>MAPLATRQGKRPSKNLKARCSRKALHVNFKDMGWDDWIIAPLEYEAFHCEGLCEFPLRSHLEPTNHAVIQTLMNSMDPESTPPTCCVPTRLSPISILFIDSANNVVYKQYEDMVVESCGCR[2x];>[2x]ETGCNKALCASDVSKCLIQELCQCRPGEGNCSCCKECMLCLGALWDECCDCVGMCNPRNYSGTLEVLFQ

Twisted gastrulation (TWSG1) is an evolutionarily conserved secreted glycoprotein which controls signaling by Bone Morphogenetic Proteins (BMPs). TWSG1 binds BMPs and their antagonist Chordin to control BMP signaling during embryonic development, kidney regeneration and cancer. TWSG1 is composed of two distinct, disulfide-rich domains. The TWSG1 N-terminal domain occupies the BMP type 1 receptor binding site on BMPs, whereas the C-terminal domain binds to a Chordin family member.

To understand how TWSG1 interacts with BMP ligands, we determined the crystal structure of the TWSG1 NTD in complex with GDF5 at 1.96 Å resolution. The disulfide-linked GDF5 dimer binds to two TWSG1 NTD molecules that are related by a non-crystallographic pseudo two-fold axis (RMSD of 0.419 Å for 138 equivalent Cα atoms of the 1:1 TWSG1 NTD:GDF5 complexes). The two TWSG1 NTD molecules in the complex adopt a similar conformation compared to the apo TWSG1 NTD (0.33 Å for 38 equivalent Cα atoms), with the major variability observed in the loop connecting helices α1 and α2. The TWSG1 NTD binds to the finger region of GDF5 and interacts with both protomers of the GDF5 dimer. The TWSG1–GDF5 interface centers around helix α1 of TWSG1 sequestered between the two finger-like motifs and helix α3 of GDF5. The side chain of TWSG1 Ile40, at the core of this interface, inserts into the hydrophobic pocket of GDF5 formed by Trp414, Trp417, Val448, Ile449, Phe478, and Tyr490, and is shielded by a salt bridge between TWSG1 Glu42 and GDF5 Lys488. TWSG1–GDF5 interactions are mediated by two salt bridges (TWSG1 Lys28-GDF5 Glu434 and TWSG1 Glu42-GDF5 Lys488), 4 hydrogen bonds, and 72 hydrophobic contacts involving 20 residues from TWSG1 and 18 residues from GDF5. Unexpectedly, the structure of the TWSG1–GDF5 complex reveals a previously unknown calcium-binding site at the edge of TWSG1–GDF5 interface. In our TWSG1–GDF5 complex, the TWSG1 NTD occupies the BMPR1-binding site on GDF5. We identified the TWSG1 NTD as the high-affinity BMP-binding domain, enabling us to determine its structure in complex with a dimeric BMP ligand. This structure revealed that TWSG1 NTD binds to the same site on BMP as BMPR1, suggesting that TWSG1 inhibits BMP signaling by competing with BMPR1 binding.> MAEFVAAQASVLIVPTLGKGANSFHQKLKEQLQTVRESVDVKIKADTAAMVAEVQATKEMLERDPINIRVETDNNGIKELVKSVTEVRHKYEDLKGDFRRGLTLNLKVVGLSALSQLGPMLASLNTSIVQLSQSSLLLPGIMSGVASSVGAAVVGSRGLTDAFKAQSDASKNVAEAGKQQRDANRAIRDSTRDLNNAIRDAKRNIEDLNAQLRDAPLDEAEAMLNLQEAQYEASQKWGKTAFQQQRDALGLAKAESQLAETRRRNVRLGQDVAEANAKGVNGNDAVVAAQERLTKALEDLAMQTGPIRALNDAMAKLSPNARDFVDQVSSLKGAWDGLRSTVQDRLFDGLGASVQTLAGQDLPILERGLAGIAGAINGNLKTAMSQLATDENKGFLGRIFGNTEEAQNRFSTALKPLLDSFMQLSAVGSDYLPRLSNAFGDVLNRFDGFIERADADGSLDKWINNGLDAMTQLGNSLINVGSIMNTISEAFTGTGGKGLLELLETGTKRLADFLKGAEGQQKLKQFFLDARTELNNWKPLLSQLPGLIKNVATAGQQWANLVLPFLTSAASLLKEHPGLVTAIFTAYMTWRTISPIIGTINL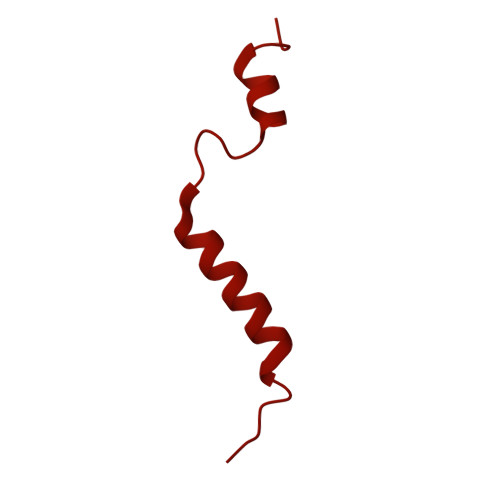LLSSETGMVGAAKKAGRAVGKGEGLTGKLGVLAGMVGQGGVVMTGLSLVAGFLINEWVTAQNEAAEAVSYHASMISRLKGEMDGLTGSLTTQGLQGKLDAARQWTDIHQTDGKPKDLVAAANSFGVDLPTFMGALTPTNQAARNAVTGKARQTVLDDLNKQGLETVLGKDALNALNLYNQNAAPDKKITNDVLADIATGVNPESKKLFEDAKKSNLIHFNESDLLYGYNKPWGFIPGTDPSGKGLSPVARDAANVSGFVLNDTGNALQVGSDIRSTNEALYGKAVLTPAGQQMFGQFGSPQASFENGSKDAAVRVDTTLQNLPPQFVKDVESNGGHFEELPDGVIIHMRKDRAAQYVTAGSYAGGGFLSGPGTGRSDSMLARVSNGEFITRAASVAKYGRGLFDALNSGTLDPSMLPRFDSGGLVDIFLPGGGTAAPPPTGSANPVDLARGLPRGPAVQSAPANRFDPSPLPTDLLPKPVIPMPDLANPGLYDPATGKYGAAPASAVQQPLKPGVDGDKGETSGPNVPPTDPRSPGYKQPNHGLGGSPGPGNGTPHLTGPGGTPVSPGAASALPSNGGIPGLTPSATDPLGLSGLPKEIQPVTILEQIGEILLSAVLGFFGLDPTYFNIGKRIFTGIKGDKPNEANPGVQSILDGYKNPLADGQNPYVGTSIYDASFDPASQRASNMAELMRGKPYTWGGSSLDGTDCSGLVMYVVDAYEGKEFSGRTGGTGGFASSLPAKGGVIISDPSQAPPGTLRVGWNASHTAGTLPDGRNFESSTFGKPIAVGAGASGYNDPQFTNWAYFPAPGYANGGFLSGAGTGRSDSMLARVSNGEFITRASSVAKYGRSLFDALNAGTVDPGMLPGFADGTPPIPGLPVPQPQTPQQAGPLPDPNGQDAQAAQQVTDTAASALDGVAGAMNGVNMGSSGAIPGADAPDGAQQGKDPRSILGAAPTNTDHNNPALSKGIQGAFSTVGSLASMAASAAMSAGTMGAGAAGASGAAGSGIQAGAQIAGQVATGALNILSSLLVGSAPGSTGTTQSAYGAPVLPQGPPQSSGGGPAVVNNYGDIHTANYDEFYKGQQRREAQQQAPILPVR>NTVTEDTPATEQAVETPQPTAVSEEAPSSSKETKIPQTPGDAEETVADDANDLAPQAPAKTADTPATSKATIRDLNDPSQVKTLQEKAGKGAGTVVAVIDAGFDKNHEAWRLTDKTKARYQSKEDLEKAKKEHGITYGEWVNDKVAYYHDYSKDGKTAVDQEHGTHVSGILSGNAPSETKEPYRLEGAMPEAQLLLMRVEIVNGLADYARNYAQAIRDAVNLGAKVINMSFGNAALAYANLPDETKKAFDYAKSKGVSIVTSAGNDSSFGGKTRLPLADHPDYGVVGTPAAADSTLTVASYSPDKQLTETATVKTDDHQAKEMPVLSTNRFEPNKAYDYAYANRGMKEDDFKDVKGKIALIERGDIDFKDKIANAKKAGAVGVLIYDNQDKGFPIELPNVDQMPAAFISRKDGLLLKDNSKKTITFNATPKVLPTASDTKLSRFSSWGLTADGNIKPDIAAPGQDILSSVANNKYAKLSGTSMSAPLVAGIMGLLQKQYETQYPDMTPSERLDLAKKVLMSSATALYDEDEKAYFSPRQQGAGAVDAKKASAATMYVTDKDNTSSKVHLNNVSDKFEVTVTVHNKSDKPQELYYQATVQTDKVDGKHFALAPKALYETSWQKITIPANSSKQVTVPIDASRFSKDLLAQMKNGYFLEGFVRFKQDPKKEELMSIPYIGFRGDFGNLSALEKPIYDSKDGSSYYHEANSDAKDQLDGDGLQFYALKNNFTALTTESNPWTIIKAVKEGVENIEAIESSEITETIFAGTFAKQDDDSHYYIHRHANGKPYAAISPNGDGNRDYVQFQGTFLRNAKNLVAEVLDKEGNVVWTSEVTEQVVKNYNNDLASTLGSTRFEKTRWDGKDKDGKVVVNGTYTYRVRYTPISSGAKEQHTDFDVIVDNTTPEVATSATFSTEDRRLTLASKPKTSQPIYRERIAYTYMDEDLPTTEYISPNEDGTFTLPEEAETMEGGTVPLKMSDFTYVVEDMAGNITYTPVTKLLEGHS[2x]

The Streptococcal C5a peptidase (ScpA) specifically inactivates the human complement factor hC5a, a potent anaphylatoxin recently identified as a therapeutic target for treatment of COVID-19 infections. The emerging view of ScpA and related subtilases is that selection of their substrates is a dynamic two-step process involving flexibility in the domains around the active site and in the C-ter of the substrate. Surface plasmon resonance (SPR) analyses of the ScpA-hC5a interaction have shown that high affinity binding of the substrate is driven by electrostatic interactions between an exosite on the Fn2 domain of the enzyme and the bulky N-ter cleavage product (PN, ’core’ residues 1-67) of C5a. ScpA, a C5a inactivating protease, represents a novel enzymatic approach to therapy.

Introduction of a D783A mutation in the Fn2 exosite, located approximately 50 Å from the catalytic serine, was shown to significantly reduce substrate binding affinity and kcat of the enzyme. X-ray crystallographic studies on the D783A mutant (ScpAD783A) were undertaken to better interpret the impact of this mutation on the specificity and activity of ScpA. X-ray diffraction data to 1.9 Å resolution were collected on a single crystal of the D783A mutant of ScpA (ScpAD783A, referred to as ‘D783A’) at the Diamond Light Source, Beamline I24. The structure was refined with PHENIX to R-work and R-free values of 19.84 and 22.89 % respectively. The data allowed for visualization of the catalytic residues and confirmed the proper folding of the enzyme. The final model includes D783A residues 97-781, 785-972, 974-995 and 999-1030. The electron density could not be assigned to three disordered regions (residues 782-784, 973 and 996-998 labelled ‘a’, ‘b’, and ‘c’ respectively in Fig. 1a). Note that the disordered regions include the D783A mutation.>[2x]MINEYFNSINDSKILSLQNKKNTLMDTSGYNAEVRVEGNVQLNPIFPFDFKLGSSGDDRGKVIVTQNENIVYNAMYESFSISFWIRINKWVSNLPGYTIIDSVKNNSGWSIGIISNFLVFTLKQNENSEQDINFSYDISKNAAGYNKWFFVTITTNMMGNMMIYINGKLIDTIKVKELTGINFSKTITFQMNKIPNTGLIT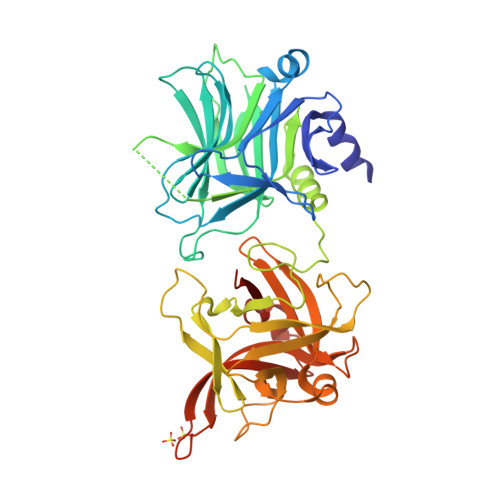SDSDNINMWIRDFYIFAKELDDKDINILFNSLQYTNVVKDYWGNDLRYDKEYYMINVNYMNRYMSKKGNGIVFNTRKNNNDFNEGYKIIIKRIRGNTNDTRVRGENVLYFNTTIDNKQYSLGMYKPSRNLGTDLVPLGALDQPMDEIRKYGSFIIQPCNTFDYYASQLFLSSNATTNRLGILSIGSYSFKLGDDYWFNHEYLIPVIKIEHYASLLESTSTHWVFVPASELEHHHHHH>TITVSTPIKQIFPDDAFAETIKANLKKKSVTDAVTQNELNSIDQIIANNSDIKSVQGIQYLPNVRYLALG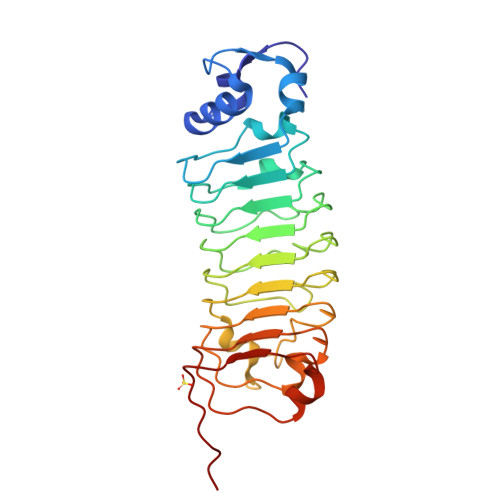GNKLHDISALKELTNLGWLNLSNNQLETLPQGVFEKLTNLTTLNLSNNQLTSLPQGVFERLASLTTLNLSNNNLANLNDKVFEGLTNLTTLNLSNNNLARLWKHANPGGPIYFLKGLTNLTTLNLSNNGFDEFPKEVFKDLTSLTTLNLSNNQLTSLPQGVFERLTNLKTLNLSNNQLQSLPTA[4x]> MVGSLNCIVAVSQNMGIGKNGDLPWPPLRNEFRYFSRMTTTSSVEGKQNLVIMGKKTWFSIPEKSRPLKGRINLVLSRELKEPPQGAHFLSRSLDDALKLTEQPELANKVDMVWIVGGSSVYKEAMNHPGHLKLFVTRIMQDFESDTFFP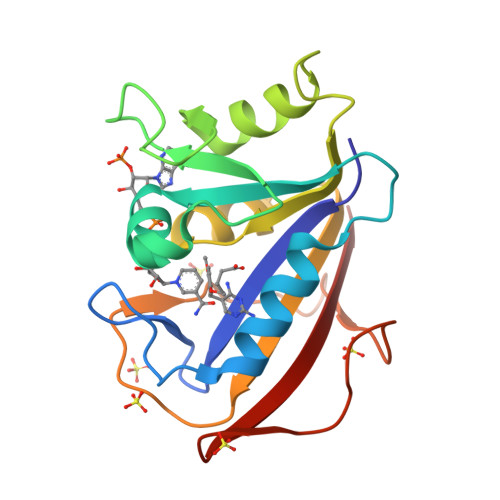EIDLEKYKLLPEYPGVLSDVQEEKGIKYKFEVYEKND> GAMADTCMSRIVKEYKVILKTLASDDPIANPYR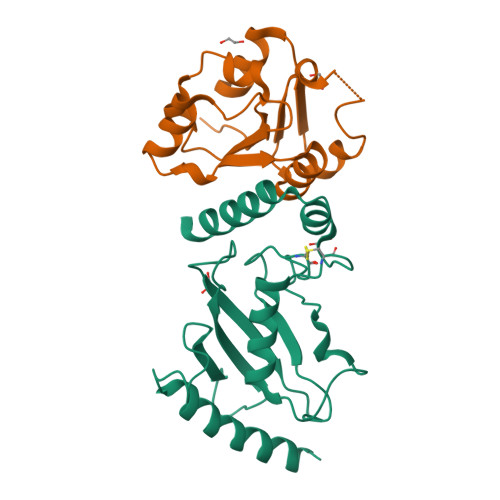GIIESLNPIDETDLSKWEAIISGPSDTPYENHQFRILIEVPSSYPMNPPKISFMQNNILHCNVKSATGEICLNILKPEEWTPVWDLLHCVHAVWRLLREPVCDSPLDVDIGNIIRCGDMSAYQGIVKYFLAERERINNH;> GAMENKKARKSKCIIMSKSIQGLPIKWEEYAADEVVLLVPTSHTDGSMKQAIGDAFRKTKNEHKIIYCDSMDGLWSCVRRLGKFQCILNSRDFTSSGGSDAAVVPEDIGRFVKFVVDSDVEDVLIDTLCN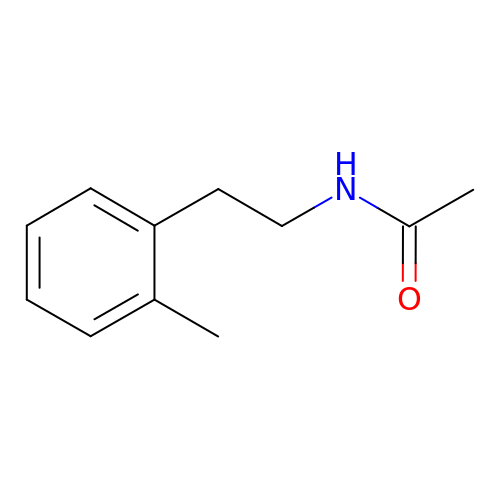~{N}-[2-(2-methylphenyl)ethyl]ethanamide | C11 H15 N O | OAMCTZZCYXDSLI-UHFFFAOYSA-N> MVSNASAL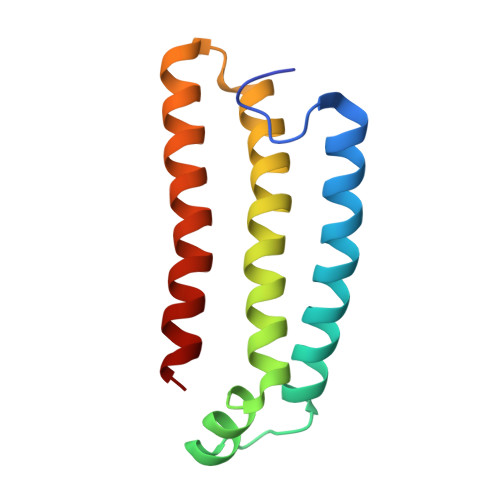GRNGVHDFILVRATAIVLTLYIIYMVGFFATSGELTYEVWIGFFASAFTKVFTLLALFSILIHAWIGMWQVLTDYVKPLALRLMLQLVIVVALVVYVIYGFVVVWGV> MDIAVQLVDSGGGTLQAGKSLRLSCAISGLAFDGGAMGSEHRLTAGAMGWFRQAPGKDREFVAAISPRTDETYYAESLEGRFSVSRDAAATMVFLQADNVRLDDTASYYCAADEDVTP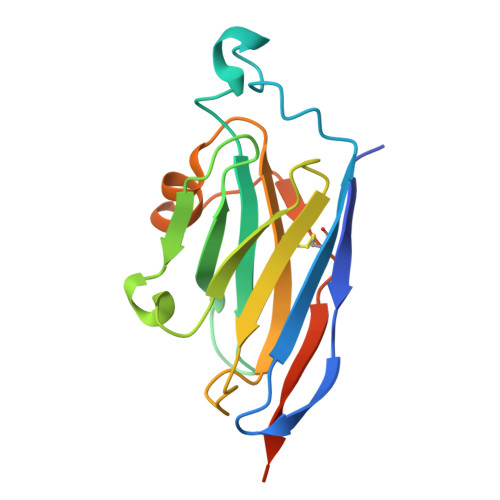RVMGVIPHADHWGQGTLVTVSSAAALEHHHHHH>QLSSNFYATKCPNALSTIKSAVNSAVAKEARMGASLLRLHFHDCFVQGCDASVLLDDTSNFTGEKTAGPNANSIRGFEVIDTIKSQVESLCPGVVSCADILAVAARDSVVALGGASWNVLLGRRDSTTASLSSANSDLPAPFFNLSGLISAFSNKGFTTKELVTLSGAHTIGQAQCTAFRTRIYNESNIDPTYAKSLQANCPSVGGDTNLSPFDVTTPNKFDNAYYINLRNKKGLLHSDQ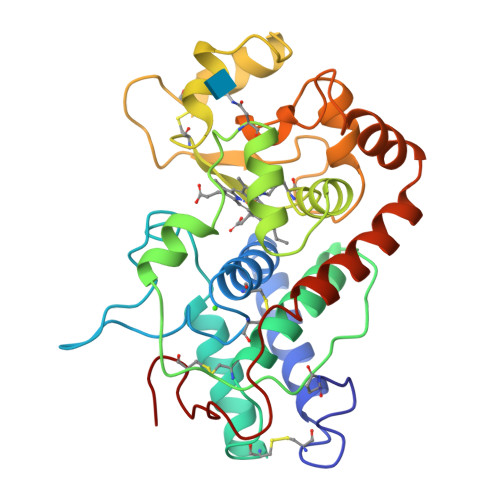QLFNGVSTDSQVTAYSNNAATFNTDFGNAMIKMGNLSPLTGTSGQIRTNCRKTN[2x]>GSHMVSKPHGGKLVNRVATEKTKEKILEEQNEFSKVQIREGTAIDLENIAHGVYSPLTGFLRKDEFQSVLDNMRLPNELPWSIPIVLDVTEKEKNFGEGDVILLYYNDTPIAKMQVDEIYTYDKKEFAKKVFKTDEEAHPGVAKTYALGEYLVGGEIELLNEVPNPFKSHTLRPVETRALFKEKGWETIVAFQTRNVPHLGHEYLQKLALTFVDGVFVNPVIGKKKKGDYKDEVILKAYETLFEHYYPKDTDILATVRYEMRYAGPREAIHHAIMRKNFGCTHFIVGRDHAGVGDYYGPYEAQEIFQNFPDLEISPIFFREFYYCKKCNAIVHDRICPHTSEYREHFSGTKIRNMIVNGELPPEYFMRKEVYETIRSFENPFVDE[2x]

Methanothermococcus thermolithotrophicus is the only known methanogen that grows on sulfate as its sole sulfur source, uniquely uniting methanogenesis and sulfate reduction. Here we use physiological, biochemical and structural analyses to provide a snapshot of the complete sulfate reduction pathway of this methanogenic archaeon. M. thermolithotrophicus activates SO42− by conventional ATPS and APSK, but transforms it further by uncanonical enzymes.

Inside the cell, SO42− is activated by an ATP sulfurylase (ATPS) to generate adenosine 5′-phosphosulfate (APS). The structure exhibits the typical ATPS fold comprising three domains (domain I, 1–156; domain II, 164–314 and domain III, 320–382). Similar to many thermophilic bacteria and archaea, the domain III contains a zinc-binding domain (320–343) that might contribute to thermal stability. All residues critical for the reaction are conserved in MtATPS, arguing for a conserved reaction mechanism.>[3x]ASNFTQFVLVDNGGTGDVTVAPSNFANGVAEWI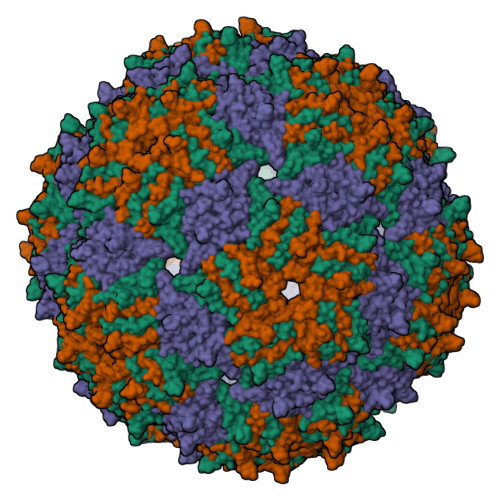SSNSRSQAYKVTCSVRQSSAQNRKYTIKVEVPKVATQTVGGVELPVAAWRSYLNMELTIPIFATNSDCELIVKAMQGLLKDGNPIPSAIAANSGIYANFTQFVLVDNGGTGDVTVAPSNFANGVAEWISSNSRSQAYKVTCSVRQSSAQNRKYTIKVEVPKVATQTVGGVELPVAAWRSYLNMELTIPIFATNSDCELIVKAMQGLLKDGNPIPSAIAANSGIY>AMKRAVITGLGIVSSIGNNQQEVLASLREGRSGITFSQELKDSGMRSHVWGNVKLDTTGLIDRKVVRFMSDASIYAFLSMEQAIADAGLSPEAYQNNPRVGLIAGSGGGSPRFQVFGADAMRGPRGLKAVGPYVVTKAMASGVSACLATPFKIHGVNYSISSACATSAHCIGNAVEQIQLGKQDIVFAGGGEELCWEMACEFDAMGALSTKYNDTPEKASRTYDAHRDGFVIAGGGGMVVVEELEHALARGAHIYAEIVGYGATSDGADMVAPSGEGAVRCMKMAMHGVDTPIDYLNSHGTSTPVGDVKELAAIR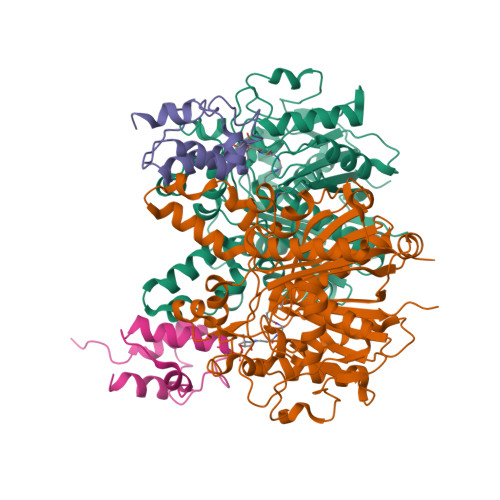EVFGDKSPAISATKAMTGHSLGAAGVQEAIYSLLMLEHGFIAPSINIEELDEQAAGLNIVTETTDRELTTVMSNSFGFGGTNATLVMRKLKD[2x];>MSTIEERVKKIIGEQLGVKQEEVTNNASFVEDLGADSLDTVELVMALEEEFDTEIPDEEAEKITTVQAAIDYINGHQA[2x]> DLGSIATWSKHAKPVACSGDWLGVRDKCFYFSDDTRNWTASKIFCSLQKAELAQIDTQED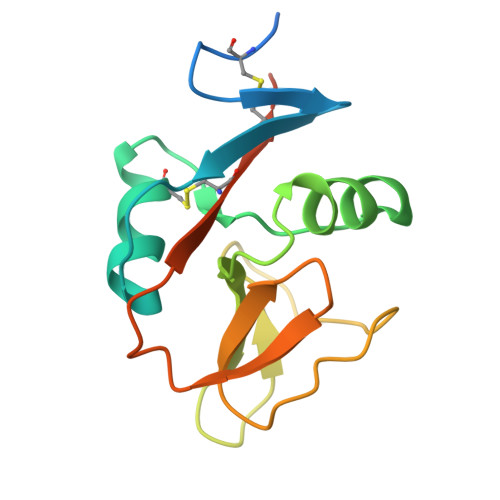MEFLKRYAGTDMHWIGLSRKQGDSWKWTNGTTFNGWFEIIGNGSFAFLSADGVHSSRGFIDIKWICSKPKYFLAAAHHHHHH> ADPGDQNPQIAAHVISEASSKTTSVLQWAEKGYYTMSNNLVTLENGKQLTVKRQGLYYIYAQVTFCSNREASSQAPFIASLCLKSPGRFERILLRAANTHSSAKPCG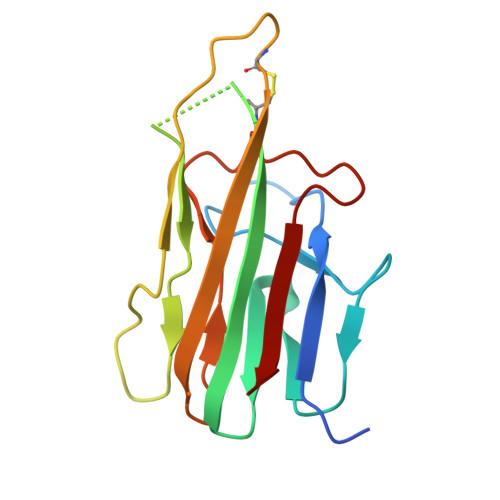QQSIHLGGVFELQPGASVFVNVTDPSQVSHGTGFTSFGLLKL> MTSNLQADMPLERIIEAEKRVECNDPLVALVVNENNTTVNNICQATHKQLFQLVQWAKLVPHFTSLPLTDQVQLLRAGWNELLIAAFSHRSMQAQDAIVLATGLTVNKSTAHAVGVGNIYDRVLSELVNKMKEMKMDKTELGCLRAIILYNPDVRGIKSV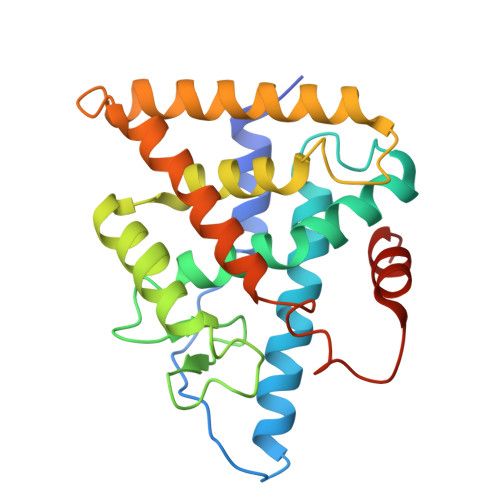QEVEMLREKIYGVLEEYTRTTHPNEPGRFAKLLLRLPALRSIGLKCLEHLFFFKLIGDVPIDTFLMEMLEGTTDS> MGSSHHHHHHSSGRENLYFQGHMGKKKNKKTEVQQPDPMRKNWIMENMDSGVIYLLESWLKAKSQETGKE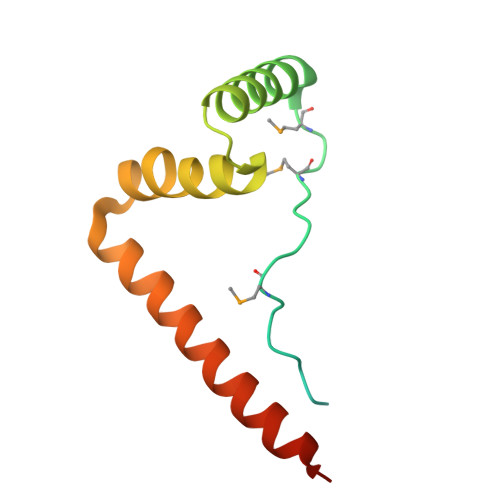ISDIFANAVEFNIVLKDWGKEKLEETNTEYQNQQRKLRKTYIEYYDREMKGS Bacteriophage Exclusion (BREX) systems recognise and methylate 6 bp non-palindromic motifs within the host genome, and prevent replication of non-methylated phage DNA that encodes these same motifs. The PglX N-terminal domain encodes the methyltransferase, whereas the C-terminal domain is for motif recognition. Our data demonstrate that PglX is used to recognise specific DNA sequences for BREX activity, contributing to motif recognition for both phage defence and host methylation. As a result, the PglX structure, and lack of nuclease motifs and potential aligned catalytic residues, supports PglX acting as a methyltransferase only, and not acting as a restriction enzyme.

Following crystallisation and data collection, an Alphafold model of PglX was used as a search model for molecular replacement, assisting the solution and refinement of the crystallographic structure of Salmonella PglX bound to S-adenosyl-L-methionine (SAM), a co-factor for methylation. The structure was refined using all data collected up to 3.5 Å. The crystal structure contains two copies of PglX in the asymmetric unit, the smallest repeating unit of the crystal. However, the arrangement of the two copies allows only weak interactions that are likely formed due to interactions within the crystal rather than being biologically significant. The architecture of PglX presents two distinct domains, N-terminal and C-terminal, linked by a central short hinge region (residues 654–659). Due to absence of available density, two short loop regions were unable to be modelled (residues 53–56 and 418–420), but otherwise the full PglX protein was resolved. Within this homologous domain of PglX (residues 227–661) sit the amino-methyltransferase motif I GxG residues implicated in SAM binding (residues 315–317), and adenine specific motif IV responsible for interacting with a flipped-out adenine base from the target DNA (NPPY; residues 509–512). PglX eluted from the SEC column at 11.2 ml, which indicated a hydrodynamic radius of 54.8 Å, matching the 57 Å calculated hydrodynamic radius of PglX. These data indicate that PglX exists as a monomer in solution, supporting our conclusions from the PglX-SAM structure.

>[2x]MNTNNIKKYAPQARNQFRDAVIQKLTTLGISADKKGNLQIADAELVGETMRYGQFDYPKSTLTRRDRLVKRAREQGFDVLVEHCAYTWFNRLCAIRYMEIHGYLDHGFHMLSHPDNPTGFEVLDHVPEVAEALLPEKKAQLVEMKLSGNQDEAIYRELLLAQCHALHRAMPFLFEAVDDEAELLLPDNLTRTDSILRGLVDGIPEEDWQEVEVIGWLYQFYISEKKDAVIGKVVKSEDIPAATQLFTPNWIVQYLVQNSVGRQWLQTYPDSPLKGKMDYYIEPAEQTPEVQAQLAAITPASIEPESIKVLDPACGSGHILIEVYNVLKNIYEERGYRARDIPQLILENNIFGLDIDDRAAQLSGFALLMMARQDDRRIFTRDVRLNIVSLQESLHLDIAKLWQQLNFHQQNQTGSMGDMFAENTALAHTDSAEYQLLMRTLKRFVNAKTLGSLIQVPQEEEAELKAFLEALYRMEQEGDFQQKAAAKAFIPYIQQAWILAQRYDAVVANPPYMGGKGMNSELKEFAKNNFPDSKADLFAMFMQNAFSLLKENGFNAQVNMQSWMFLSSYEALRNWLLDNKTFITMAHLGARAFGQISGEVVQTTAWVIKNQHSERYQPVFFRLIDGREEVKKSDLLLRKNIFDKFTQHDFKNIPGMPIAYWIDLPSLLSFRHHKKLGEKIALKAGMSTGDNIKFQRYWYEVSIKKTLITNKESNTKIDIHNIKWFPCSSGGEYRKWYGNNEIVVNWENNGYEIRNFKFENGKTRSAVRNDEYYFREGITWSKISQGNFCVRYRPKGFVFDDTGRCGFSNNKNELLYAAGLMCTPVVNHYLSILAPTLSFTSGELASVPYPEIEDEIIELVTNAIEIAKNDWDSQEQSWDYVCSPLLEHNSTQLLRNIYKQKINTNIKLVETLLLIENTINNIFIDKLQLDKTIIKAVLQSEITLLCNPNYRYKNIQDHTDLTNKYYTDITIDILSYIIGCMMGRYSLDREGLVYAHEGNKGFAELVAEDAYKTFPADNDGILPLMDDEWFDDDVTSRVKEFVRTVWGEEHLQENLEFIAESLCLYAIKPKKGESALDTIRRYLSTQFWKDHMKMYKKRPIYWLFSSGKEKAFECLVYLHRYNDATLARMRTEYVVPLLARYQANIDRLNEQVDGASGGEATRLKRERDSLSKKFNELRSFDDRLRHYADMRISIDLDDGVKVNYGKFGDLLADVKAITGNAPEII>MKYILVTGGVISGIGKGIIASSIGTILKSCGLRVTAIKIDPYINIDAGTFSPYEHGEVFVLNDGGEVDLDLGNYERFLDINLYKDNNITTGKIYQHVINKERRGDYLGKTVQVVPHITDAIQEWVMNQAKVSVDGNKEDPQICVIELGGTIGDIEGMAFVEAFRQFQFKAKKENFYNIHVSLVPQPSATGEQKTKPTQNSVRALRGLGLSPDLIVCRSSTPIEMAVKEKISMFCHVNPEQVICIHDVSSIYRVPLLLEEQGVVKYFQERLGLPINDCSSNLLFKWKAMADRYERLQKICSIALVGKYTKLRDCYASVFKALEHSALAINHKLNLMYIDSIDLEP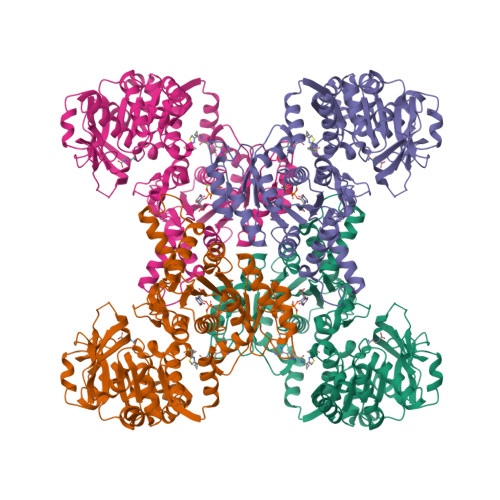VTKAEDPVKFHEAWQKLCLADGILVPGGFGIRGTLGKLQAISWARTKKIPFLGICLGMQLAVIEFARNCLNLKDANSTEFEPNTPVPLVIDMPEHNPGDLGGTMRLGLRRTVFTTENSILKKLYGDVPYIEERHRHRYEVNPNLINQFENKDLCFVGEDVDGKRMEIVELTSHPYFIGVQFHPEFSSRPMKPSPPYLGLLLAATGNLNAHLQQMNKLPYSDGYSDASDDSFPEAKLAELDLN[4x]> MSITLRTYIFLDALQPQLATFIGKTARGFLPVPGQASLWVEIAPGIAINRVTDAALKATKVQP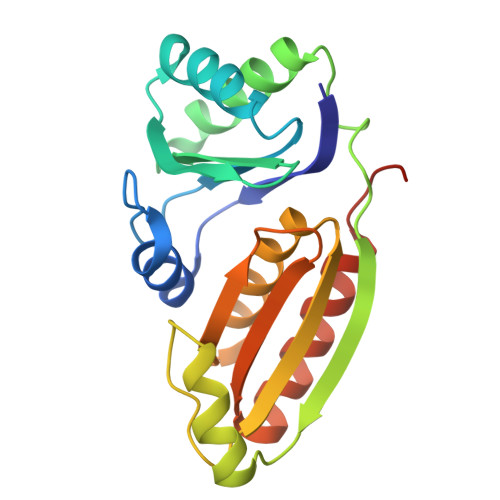AVQVVERAYGLLEVHHFDQGEVLAAGSTILDKLEVREEGRLKPQVMTHQIIRAVEAYQTQIINRNSQGMMILPGESLFILETQPAGYAVLAANEAEKAANVHLVNVTPYGAFGRLYLAGSEAEIDAAAEAAEAAIRSVSGVAQESFRDR>MSLKNQLGQLALEQAKTFGGKLEVQPKVDIKTKHDLSIAYTPGVASVSSAIAKDKTLAYDLTTKKNTVAVISDGTAVLGLGDIGPEAAMPVMEGKAALFKAFAGVDAIPIVLDTKDTEEIISIVKALAPTFGGINLEDISAPRCFEIEQRLIKECHIPVFHDDQHGTAIVVLAAIFNSLKLLKKSLDEVSIVVNGGGS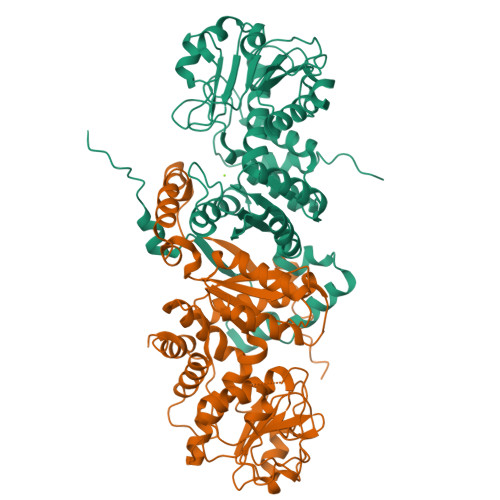AGLSITRKLLAAGATKVTVVDKFGIINEQEAAQLAPHHLDIAKVTNREFKSGTLEDALEGADIFIGVSAPGVLKAEWISKMAARPVIFAMANPIPEIYPDEALEAGAYIVGTGRSDFPNQINNVLAFPGIFRGALDARAKTITVEMQIAAAKGIASLVPDDALSTTNIIPDAFKEGVAEIVAKSVRSVVLKSEGHHHHHH[2x]N-[1-(AMINOMETHYL)CYCLOPROPYL]-3-(BENZYLSULFONYL)-N~2~-[(1S)-2,2,2-TRIFLUORO-1-(4-HYDROXYPHENYL)ETHYL]-L-ALANINAMIDE 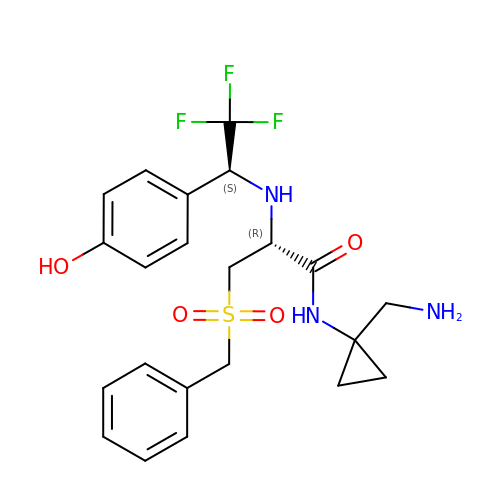| C22 H26 F3 N3 O4 S | DWWVPKCSDHDILN-OALUTQOASA-N> EPEQD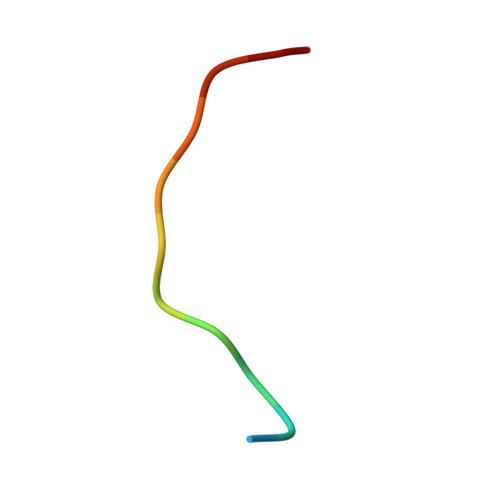SAVTSGE>MPIPNNPGAGENAFDPVFVNDDDGYDLDSFMIPAHYKKYLTKVLVPNGVIKNRIEKLAYDIKKVYNNEEFHILCLLKGSRGFFTALLKHLSRIHNYSAVETSKPLFGEHYVRVKSYCNDQSTGTLEIVSEDLSCLKGKHVLIVEDIIDTGKTLVKFCE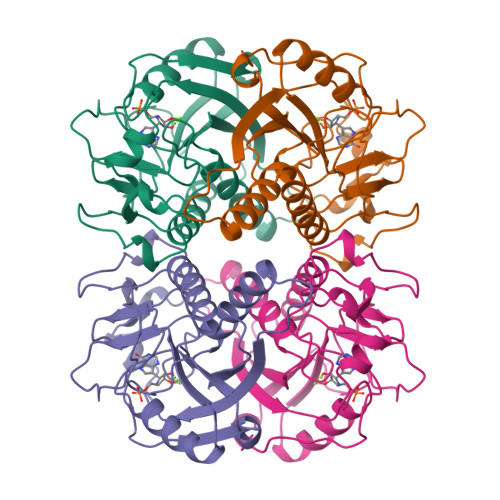YLKKFEIKTVAIACLFIKRTPLWNGFKADFVGFSIPDHFVVGYSLDYNEIFRDLDHCCLVNDEGKKKYKATSL[4x]>GPGADRAQDHNNNNTPRNSNYVVEEEEVSEEEEEAIMMPDFGDHVDTSIFGQILEMDEGDDHDFSAPLVLNFFEQAEETFQKMETALNNKDLPELSKLGHFLKGSSATLGFTKIRDSCQLIQQYGHGLNVDGSSEPDEGVCLKKIAEALASAAVDTVALHKMMREFFEY[2x]

If the HK incorporates a REC domain (REC-1) is denoted as hybrid histidine kinase (hHK), and the first His-Asp phosphotransfer event occurs in the same polypeptide chain. Then, HPt protein containing a phosphorylatable His shuffles the phosphoryl group from the phosphorylatable Asp in the REC-1 domain to the phosphorylatable Asp in the REC domain of an RR (REC-2) in two more phosphotransfer steps. In fungi, the HPt accepts the phosphoryl group from REC-1 domains of various hHKs upstream of the signaling pathway and forwards it downstream to REC-2 domains present in at least two conserved RRs, Ssk1 and Skn7. Also, we have obtained the crystal structures of Ct_HPt alone and in complex with REChHK6 bound to the phosphomimetic BeF3−, as well as the crystal structures of REChHK3 and RECCa_Sln1.

However, to assess the impact on protein stability of the residues involved in salt bridge formation, we produced single mutants E82A, E89A, R158A, R169A, and a double mutant R158A/E82A. A thermal shift assay revealed changes in the thermal denaturation temperature (Tm) only for R158A and R158A/E82A which dropped to 54 °C in comparison with the Tm of 61.5 °C for the WT. Also, SEC analysis for the mutants showed a change in their elution profile in comparison with the WT, with a second peak eluting at a lower volume. However, SEC-MALS analysis with mutant R158A identified a single monomeric species in solution with a MW of 19.9 kDa similar to WT. Thus, the salt bridges involving R158 seemed to play a relevant role in the stability of the helix bundle. We determined the structure of the mutant R158A, albeit at a low resolution of 3.4 Å, observing two molecules in the AU with no differences in the helix bundle with respect to the WT (rmsd ~0.6 Å for 128 residues) but in the crystal packing. The absence of R158 changed the electrostatic nature of the interface and allowed the approach of αE in both molecules to a distance of ~4 Å between Cα of A155–A155.Staphylococcus aureus FakB1 is a prototypical bacterial FA transfer protein that binds palmitate within a narrow, buried tunnel. Here, we use a combination of X-ray crystallography, NMR spectroscopy, MD simulations, site-directed mutagenesis, and functional biochemical assays to characterize the membrane-bound conformation of FakB. This study focuses on FakB1, an FA transfer protein from S. aureus that binds palmitic acid (16:0) before presenting it to FakA for phosphorylation and exchange with the membrane. The bacterial class of FA transfer proteins is called FakB, and the bound acyl chains are completely enclosed within the protein interior. The open conformation arises from a conformational change in the dynamic region that rotates helix α8 outward to uncover the FA-binding tunnel and reorganizes the adjacent α8-β9 loop into a new amphipathic helix.

We identified two alanine residues (121 and 158) in the tunnel and mutated them to bulkier residues to partially occlude the FA-binding pocket and push the FA out of its pocket to destabilize the fully closed FakB1 conformation. The 2.35 Å crystal structure of the FakB1(A121I, A158L) double mutant was also determined, and superposition of the FakB1(A121I) and FakB1(A121I, A158L) structures shows that they are basically identical with an RMSD = 0.241 Å. Thus, three independent mutants generated the identical conformational change.

>HMKIAVMTDSTSYLSQDLIDKYNIQIAPLSVTFDDGKNFTESNEIAIEEFYNKMASSQTIPTTSQPAIGEWITKYEMLRDQGYTDIIVICLSSGISGSYQSSYQAGEMVEGVNVHAFDSKLIAMIEGCYVLRAIEMVEEGYEPQQIIDDLTNMREHTGLYLIVDDLKNLQKSGRITGAQAWVGTLLKMKPVLKFEDGKIIPEEKVRTKKRAIQTLEKKVLDIVKDFEEVTLFVINGDHFEDGQALYKKLQDDCPSAYQVAYSEFGPVVAAHLGSGGLGLGYVGRKIRLT[2x]>[35x]MNHKVHHHHHHIEGRHMADKSTDLTVTEGGSDGALVASSDVDVESQNPDLEERSASKFDMAVGDLDLLRQVVLVLSISICVALIVMLFFWVKEPEMRPLGAYETEELIPVLDYLDQQKINYKLDGNTISVESSEYNSIKLGMVRSGVNQATEAGDDILLQDMGFGVSQRLEQERLKLSRERQLAQAIEEMKQVRKARVLLALPKHSVFVRHNQEASASVFLTLSTGTNLKQQEVDSIVDMVASAVPGMKTSRITVTDQHGRLLSSGSQDPASAARRKEQELERSQEQALREKIDSVLLPILGYGNYTAQVDIQMDFSAVEQTRKRFDPNTPATRSEYALEDYNNGNMVAGIPGALSNQPPADASIPQDVAQMKDGSVMGQGSVRKESTRNFELDTTISHERKQTGTVARQTVSVAIKDRRQVNPDTGEVTYTPMSESEINAIRQVLIGTVGFDQGRGDLLNVLSVKFAEPEAEQLEEPPIWEHPNFSDWVRWFASALVIIVVVLVLVRPAMKKLLNPTSDDEDEMYGPDGLPIGADGETSLIGSDIESSELFEFGSSIDLPNLHKDEDVLKAVRALVANEPELAAQVVKNWMNDMANDIVPQDDNAAGMPVELDVSTITGEEKAAILLLSLNEQDAAGIIRHLEPKQVQRVGSAMAKAKDLSQDKVSAVHRAFLEDIQKYTNIGMGSEDFMRNALVAALGEDKANNLVDQILLGTGSKGLDSLKWMDPRQVASIIVNEHPQIQTIVLSYLEADQSAEILSQFPERVRLDLMMRIANLEEVQPSALAELNEIMEKQFAGQAGAQAAKISGLKAAAEIMNYLDNNVEGLLMEQIRDQDEDMATQIQDLMFVFENLVEVDDQGIQKLLRDVPQDVLQKALKGADDSLREKVFKNMSKRAAEMMRDDIEAMPPVRVADVEAAQKEILAIARRMADAGELMLSGGADEFL

The C-ring is tightly attached to the MS-ring, which consists of ~34 FliF molecules with two transmembrane helices. FliF contains three ring-building motifs (RBM1, RBM2, and RBM3) and β-collar in the periplasmic region between the two transmembrane helices. Among these motifs, RBM3–β-collar forms an S-ring on the distal side of the cytoplasm within the MS-ring. We performed single-particle cryo-EM of the purified MS-ring formed by FliFG fusion proteins with the FliG-G214S mutation and determined the near-atomic resolution structure of the Vibrio S-ring.

A total of 228,461 particle images extracted from 5,962 cryo-EM micrographs were analyzed. They were separated into two classes in the 2D class averages, with them showing either 35- or 34-fold rotational symmetry on the S-ring. No other symmetry in the 2D class averages was observed, indicating that the purified MS-ring consisted of 35 or 34 subunits of the FliFG fusion proteins, and there was no other variation. Because the MS-ring in the native flagellar motor is thought to comprise 34 FliF subunits, it is inferred that the 34-fold rotational symmetry structure reflects the native S-ring structure, whereas the 35-fold rotational symmetry structure is an artificial structure induced by the overexpression of FliFG fusion proteins alone. After postprocess without symmetry correction, their resolutions of 35 and 34 subunit MS-rings were 3.76 and 4.28 Å, respectively. Consequently, we built the atomic model of the S-ring part (RBM3–β-collar) at 3.23 and 3.33 Å resolutions from the maps of both classes after C35 and C34 rotational symmetry corrections, respectively. The monomeric structures in the S-ring part from the 35- and 34-mer structures are almost identical (RMSD = 0.286 Å). Our S-ring structures are composed of 34 or 35 molecules of the FliFG fusion protein. Their diameters differ: the outer and inner diameters are about 26.0 nm and 9.6 nm, respectively, in the 35-mer ring, and about 25.2 nm and 9.4 nm, respectively, in the 34-mer ring. The difference in the outer and inner circumferences derived from these diameters is approximately 2.4 nm and 0.7 nm, respectively, which are roughly equal to the calculated differences produced by one subunit.>[4x]GPGMLSVLLCTSSSYQTQTIGRLTTPGTNLVKAYKTSNPDLNRNCYWLYFDYYVHILGYENGFAHVRIGTEDCWISKDSLEEITIPTKSVTEANIYSEPSRAETIIRYVPANSDVTILDFNCDGFYRINYRGYIGYILEDALQYKWKQVDGANDGERAANLVKTKLGCKYVWAMSGPDTFDCSGLMQWAYNRLDIFMHRTADVQGNHGQLIEDAKDILPGDIITFHTDSEKPTAVTHV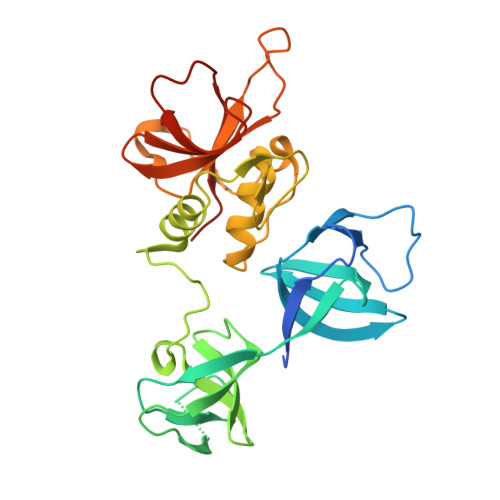GMYVGNGQFIHASTNGYVVRYQDFNSYPYPVSSIRRYWTK>QVVIGPGDRPETGLQGQTTIEDVVSGRSKLPYHAGVRLVGRTDIWNRGGNLQLSWVDQCAYVSTFKQAGPITANSRSALFLREPAGVAVIDVRDPRAPKPVRLLRDRGSIDAVETMHAIAAPGRKVLVAGAYSGGIAGRGEEDAAWLSIYDASNCLNPKLQSEFKWPANIHMVTISPNGRRVYGTEVVPGLGSGKGGLHVLDISDMKRPRYLGRFGVTRPNGLTAGFTPHEVSISHDERRIYAAVLASETGDVPVGASILASDGDVPVENGSVYILDNSDIVDGRSQPKMRLVGEAKQGGFHSVVPASINGVPHLVGAAELGACPGTWPRIINIADEKNPKIVGEFKLQMNIKENCDAIRFTPRKEDPYASFIPIPDITA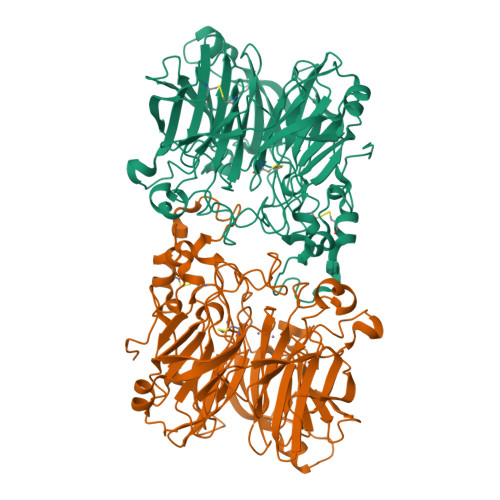RLGAVGSHFNDVDDARNTRLGLFPFFAGGVRIVDLRDPTKPVEVGYYKPGANPDTPLSGNGLNWTGLNDQVTDGCMSHVRYVPESGHIWFACVTTGFHVVELNPDLRARLGFPTVKLEHHHHHH[4x]>[4x]MEFRQLKYFIAVAEAGNMAAAAKRLHVSQPPITRQMQALEADLGVVLLERSHRGIELTAAGHAFLEDAR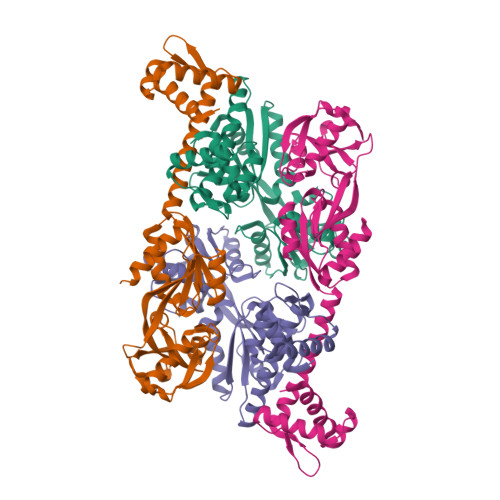RILELAGRSGDRSRAAARGDVGELSVAYFGTPIYRSLPLLLRAFLTSTPTATVSLTHMTKDEQVEGLLAGTIHVGFSRFFPRHPGIEIVNIAQEDLYLAVHRSQSGKFGKTCKLADLRAVELTLFPRGGRPSFADEVIGLFKHAGIEPRIARVVEDATAALALTMAGAASSIVPASVAAIRWPDIAFARIVGTRVKVPISCIFRKEKQPPILARFVEHVRRSAKD(2R)-2-[4-(aminomethyl)benzyl]-3-[(R)-[(1R)-1-amino-3-phenylpropyl](hydroxy)phosphoryl]propanoic 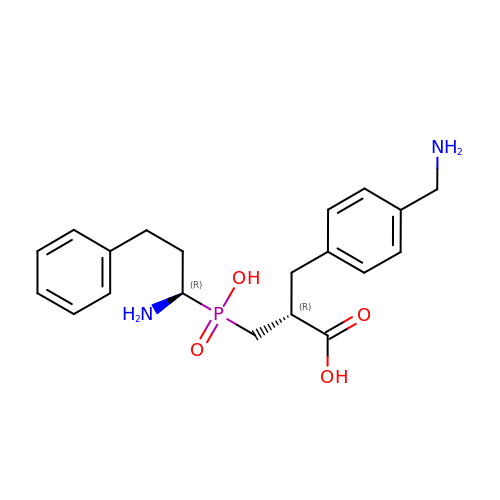acid | C20 H27 N2 O4 P | XZFPYKBNMOQQLL-RBUKOAKNSA-N>GRSNMGKLKQEMGGIVTELIRDYQSSREDSLQDAWDYVQAQVKCCGWVSFYQWTDNAELMNRPEVTYPCSCEVKGEEDNSLSV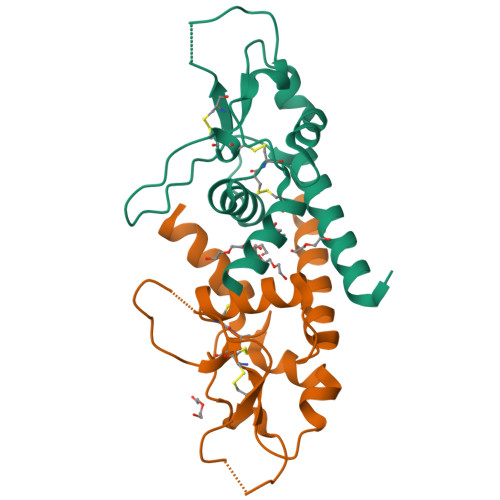RKGFCEAPGQRTQSGNHPEDWPVYQEGCMEKVQAWLQENL[2x]> NDDKLYRADSRPPDEIKQSGGLMPRGQSEYFDRGTQMNINLYDHARGTQ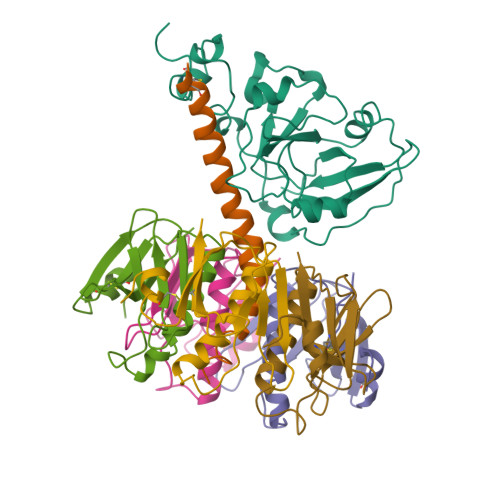TGFVRHDDGYVSTSISLRSAHLVGQTILSGHSTYYLYVLATAPNMFNVNDVLGAYSPHPDEQEVSALGGIPYSQIYGWYRVHFGVLDEQLHRNRGYRDRYYSNLDIAPAADGYGLAGFPPEHRAWREEPWIHHAPPGCGNAPRSS;> MSNTCDEKTQSLGVKFLDEYQSKVKRQIFSGYQSDIDTHNRIKDEL;>[5x]TPQNITDLCAEYHNTQIYTLNDKIFSYTESLAGKREMAIITFKNGAIFQVEVPSSQHIDSQKKAIERMKDTLRIAYLTEAKVEKLCTWNNKTPHAIAAISMAN> GPAAMSGSIPEIYLDVVTKETISDKYKDWHFISKNCHYEQLMDLEMKDTAYSFLFGSSRSQGKVPEFVHLKCPSITNLLVLFGVNQEKCNSLKINYEKKENSRYDNLCTIFPVNKMLKFLMYFYSDDDNDDVREFFLKAFICLILDRKVFNAMESDHRLCFKVLELFNEAHFINSYFEIVDKNDFFLHYRLLQIFPHLQSALLRRRFSEKQGRTETIQQNIIKEFNEFFDCKNYKNLLYFILTMYGSKFIPFGPKCQVTEYFKDCILDISNETTNDVEISILKGILNLFSKIRGXXXXXXXXXXXXXX;> MDGALINSVLYVSPRNGAHYFVELTEKHLLAFEMLNSMCLLENYDHVLLFLECQFGKSHNLAVIPFDIILVLFTLSTLSEYYKEPILRANDPYNTSRETLSRRALKLLQKYLAILKEFDSEQYNLYDLELLRCQFFLAIDTLTPKKQKWGFDRFRRTKSESGVTYRQNASVDPELDQAKTFKNPYRSYISCLEQRNTILGNRLLNLKLNEPGEFINMILWTLSNSLQESTPLFLSSHEIWMPLLEILIDLFSCRQDYFIQHEVAQNVSKSLFVQRLSESPLAVFFESLNTRNFANRFSEYVFLNCDYKLPSDNYATPVHPVYNGENTIVDTYIPTIKCSPLYKSQKSLALRRKLIGSCFKLLLRVPDGHRLITPRIVADDVIQGISRTLASFNDILQFKKFFMTENLSQESYFIPLLAEGTLSEILKDTQECVVILTLVENLSDGVSFCNEVIGLV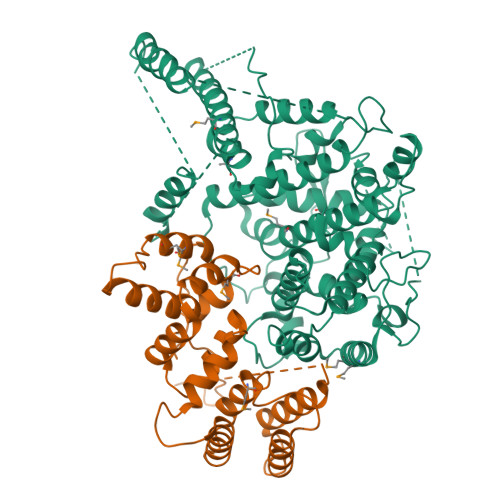KSKCFAFTEQCSQASYEEAVLNIEKCDVCLLVLLRYLLHLIGTEAILDAKEQLEMLHAIEKNDSGRRQWAKALNLGNDPPLLYPIVSQMFGVHDKSVIIEXXXXXXXXXXXXXXXXXXXXXXXXXXXXXXXXXXXXXXXXXXXXXXXXXXX>MRKQLAQIKEMVELPLRHPALFKAIGVKPPRGILLYGPPGTGKTLIARAVANETGAFFFLINGPEIMSKLAGESESNLRKAFEEAEKNAPAIIFIDELDAIAPKREKTHGEVERRIVSQLLTLMDGLKQRAHVIVMAATNRPNSIDPALRRFGRFDREVDIGIPDATGRLEILQIHTKNMKLADDVDLEQVANETHGHVGADLAALCSEAALQAIRKKMDLIDLEDETIDAEVMNSLAVTMDDFRWALSQSNPSALRETVVEVPQVTWEDIGGLEDVKRELQELVQYPVEHPDKFLKFGMTPSKGVLFYGPPGCGKTLLAKAIANECQANFISIKGPELLTMWFGESEANVREIFDKARQAAPCVLFFDELDSIAKARGGNIGDGGGAADRVINQILTEMDGMSTKKNVFIIGATNRPDIIDPAILRPGRLDQLIYIPLPDEKSRVAILKANLRKSPVAKDVDLEFLAKMTNGFSGADLTEICQRACKLAIRESIESEIRRERERQTNPSAMEVEEDDPVPEIRRDHFEEAMRFARRSVSDNDIRKYEMFAQTLQQSRGFGSFRFPSGNQGGAGPSQGSGGGTGGSVY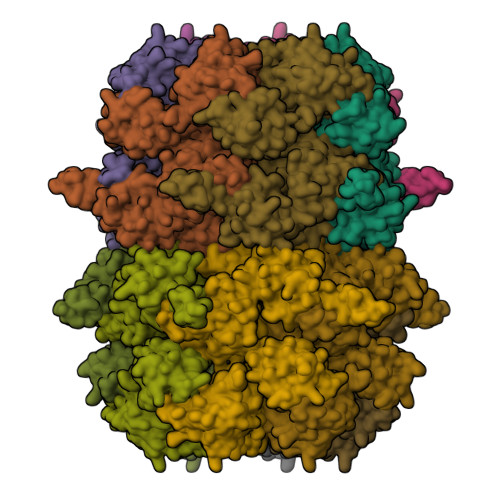TEDNDDDLYGRSHHHHHH[12x]>MCDQFVGTWKFLSSENFEDYMKELGVGFATRKMAGVAKPNVTISINGDVITIKTESTFKNT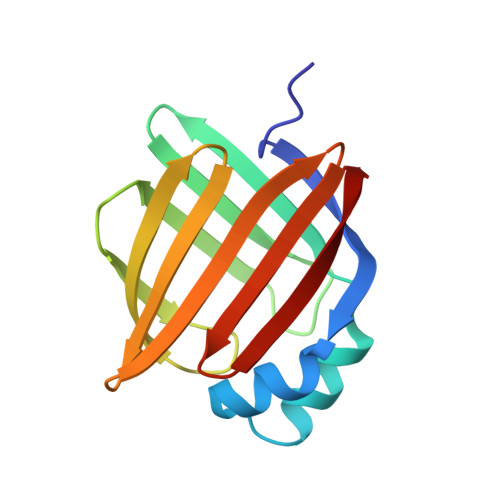EVSFRLGEEFDETTADDRKTKNVITLDNGILNQVQKWDGKETVIKRKVMDGNLVVECTMNTVTSKRVYERA[2x]> DPFTQFKQTPLPYAYDALEGAIDAKTMEIHYSKHHAGYTANLNKAIAGTPAEKESIENILAKVSQYSDAVRNNAGGHYNHELFWSILTPNKGTKPSAALQKAIDETFGSLDALKEKINAAGAARFGSGWAWLIVDN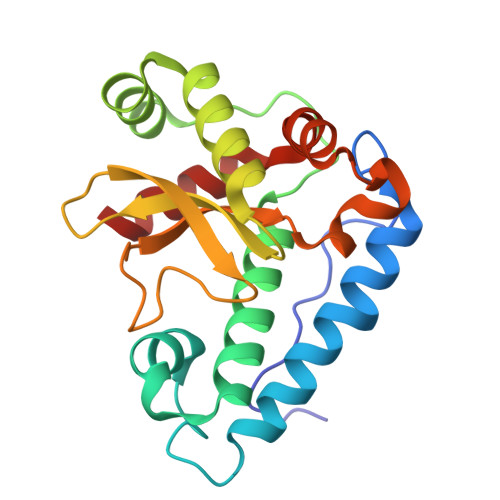GGKLQVTSTPNQDNPLMDFTKEKGTPILGIDVWEHAYYLRYQNKRADYLTTIWDVINWEEVSARYEKAL>MMFGKKKNNGGSSTARYSAGNKYNTLSNNYALSAQQLLNASKIDDIDSMMGFERYVPPQYNGRFDAKDIDQIPGRVGWLTNMHATLVSQETLSSGSNGGGNSNDGERVTTNQGISGVDFYFLDEEGGSFKSTVVYDPYFFIACNDESRVNDVEELVKKYLESCLKSLQIIRKEDLTMDNHLLGLQKTLIKLSFVNSNQLFEARKLLRPILQDNANNNVQRNIYNVAANGSEKVDAKHLIEDIREYDVPYHVRVSIDKDIRVGKWYKVTQQGFIEDTRKIAFADPVVMAFDIETTKPPLKFPDSAVDQIMMISYMIDGEGFLITNREIISEDIEDFEYTPKPEYPGFFTIFNENDEVALLQRFFEHIRDVRPTVISTFNGDFFDWPFIHNRSKIHGLDMFDEIGFAPDAEGEYKSSYCSHMDCFRWLKRDSYLPQGSQGLKAVTQSKLGYNPIELDPELMTPYAFEKPQHLSEYSVSDAVATYYLYMKYVHPFIFSLCTIIPLNPDETLRKGTGTLCEMLLMVQAYQHNILLPNKHTDPIERFYDGHLLESETYVGGHVESLEAGVFRSDLKNEFKIDPSAIDELLQELPEALKFSVEVENKSSVDKVTNFEEI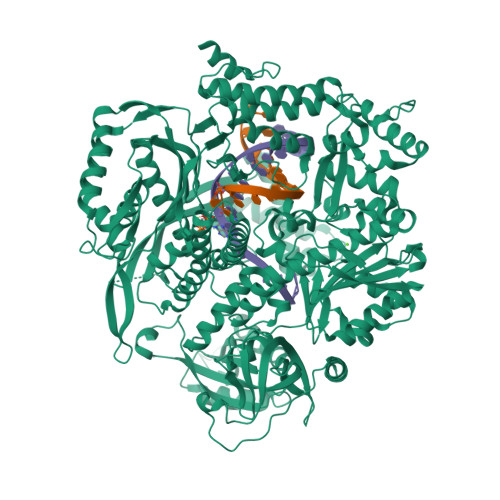KNQITQKLLELKENNIRNELPLIYHVDVASMYPNIMTTNRLQPDSIKAERDCASCDFNRPGKTCARKLKWAWRGEFFPSKMDEYNMIKRALQNETFPNKNKFSKKKVLTFDELSYADQVIHIKKRLTEYSRKVYHRVKVSEIVEREAIVCQRENPFYVDTVKSFRDRRYEFKGLAKTWKGNLSKIDPSDKHARDEAKKMIVLYDSLQLAHKVILNSFYGYVMRKGSRWYSMEMAGITCLTGATIIQMARALVERVGRPLELDTDGIWCILPKSFPETYFFTLENGKKLYLSYPCSMLNYRVHQKFTNHQYQELKDPLNYIYETHSENTIFFEVDGPYKAMILPSSKEEGKGIKKRYAVFNEDGSLAELKGFELKRRGELQLIKNFQSDIFKVFLEGDTLEGCYSAVASVCNRWLDVLDSHGLMLEDEDLVSLICENRSMSKTLKEYEGQKSTSITTARRLGDFLGEDMVKDKGLQCKYIISSKPFNAPVTERAIPVAIFSADIPIKRSFLRRWTLDPSLEDLDIRTIIDWGYYRERLGSAIQKIITIPAALQGVSNPVPRVEHPDWLKRKIAT[2x]~{N}-[(1~{R})-1-[3-azanyl-5-(trifluoromethyl)phenyl]ethyl]-6,7-dimethoxy-2-methyl-quinazolin-4-amine 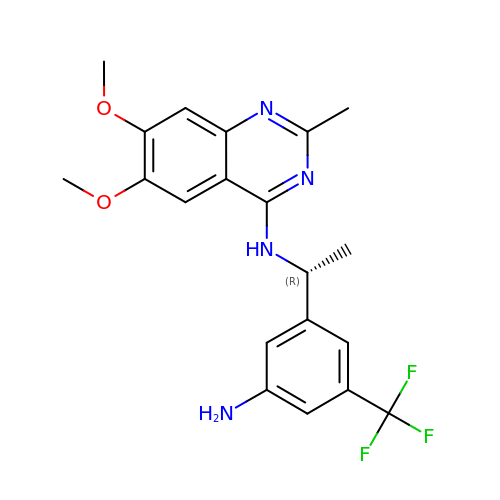| C20 H21 F3 N4 O2 | UCSYKUAZQWUWGJ-SNVBAGLBSA-N>[4x]GSELTEDEEEMVEKILKAHEETFPYLTDDDKYRLTQEELEKGNVILWERVSELSTKAIANVVDFGKQVPVFTQLSTNDQITLLK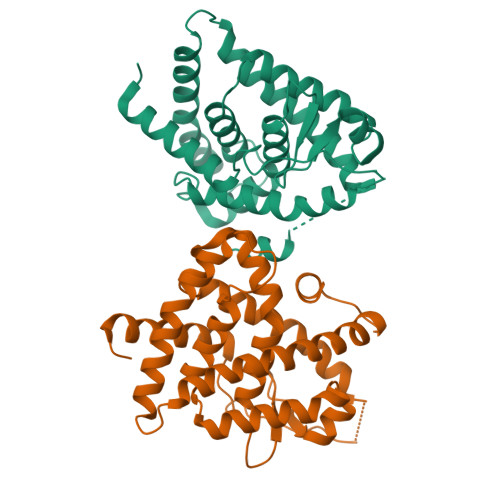AACLEIIILRLASRYDDKEDTMSFSNGLTLTQQQLEVGGFGTLTPTIFKFARSLVELSVDTAEYAMLSLICLISGDRSGLEHPEKVEQKQEPILETLKHYVRKRRPDSPHSFAKLLLKLTDLRSLSVKGAERVLQLRMEMPGELPPLILEMLDRTEN> PLSPPTNLHLEANPDTGVLTVSWERSTTPDITGYRITTTPTNGQQGNSLEEVVHADQSSCTFDNLSPGLEYNVSVYTVKDDKESVPISDTII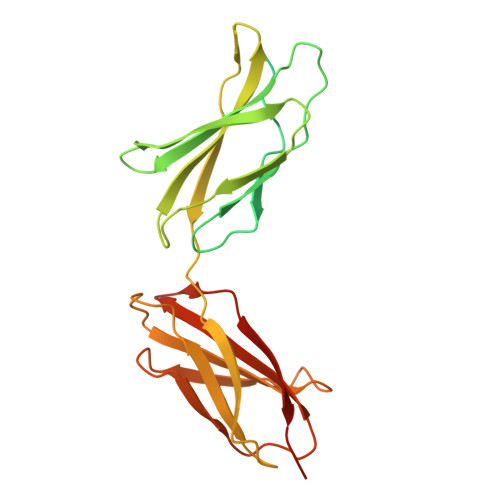PEVPQLTDLSFVDITDSSIGLRWTPLNSSTIIGYRITVVAAGEGIPIFEDFVDSSVGYYTVTGLEPGIDYDISVITLINGGESAPTTLTQQTAVPPPTDLRFTNIGPDTMRVTWAPPPSIDLTNFLVRYSPVKNEEDVAELSISPSDNAVVLTNLLPGTEYVVSVSSVYEQHESTPLRGRQKTGSAHHHHHH>GSPSKTKSAPVSYDKDGMNASEEDFSFDNTLAKPYEPLYARRGDITSAGSTSGEDSSQPKMITISGEQLNLITENKELMNELTLVSTELAESI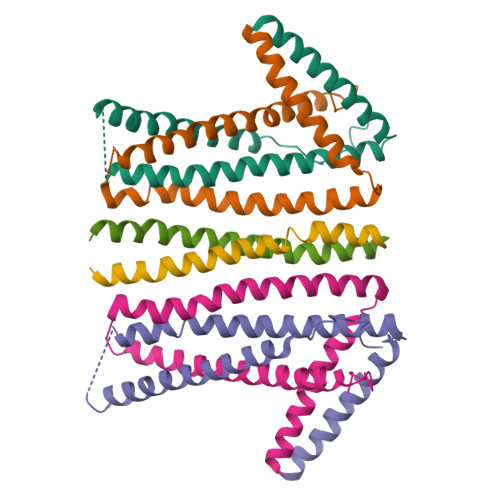KRETELEERIRLYETNNSAPSFDDSSSVSFSDFEKELRKKSSKIVQLIQQLNDERLKRFIAEEQLLLQENGTKPSSMELVGRIENLNKLIDERDSEIEMLKGRLQ[4x];>MTDNLTTTHGGSTTLELLAQYNDHRSKKDKSIEHIEKGTCSGKERNPSYDEIFTENIKLKLQVQEYETEIESLEKVIDMLQKNREASLEVVLEQVQNDS[2x]Ribosomal RNA synthesis in Escherichia coli involves a transcription complex, in which RNA polymerase is modified by a signal element on the transcript, Nus factors A, B, E and G, ribosomal protein S4 and inositol mono-phosphatase SuhB. This complex is resistant to ρ-dependent termination and facilitates ribosomal RNA folding, maturation and subunit assembly. We show that SuhB directly binds the RNA signal element and the C-terminal AR2 domain of NusA, and we delineate the atomic basis of the latter interaction by macromolecular crystallography. The SuhB monomers are folded as an alternating stack of three pairs of α helices (helix pairs I–III) and two β sheets.

About 1600 Å2 of combined surface area are buried at the dimer interface. It has been suggested that wild type (wt) SuhB might form monomers, and that the R184A mutation stabilized the dimer state observed in the crystal structure of SuhBR184A. We therefore also crystallized wt SuhB alone and determined its structure at 2.25 Å resolution. Isolated wt SuhB crystallized with one monomer in an asymmetric unit, but a dimer essentially identical to the dimer seen with SuhBR184A (rmsd 0.56 Å for 482 pairs of common Cα atoms) and in the SuhB-NusAAR2 complex (rmsd 0.49 Å for 497 pairs of common Cα atoms) was formed by crystal symmetry. Moreover, SEC coupled to multi-angle light scattering confirmed that SuhB forms dimers under the chosen conditions in solution (experimental molecular mass: 60.7 kDa; calculated molecular mass for a SuhB dimer: 58.3 kDa).

> GAMAMHPMLNIAVRAARKAGNLIAKNYETPDAVEASQKGSNDFVTNVDKAAEAVIIDTIRKSYPQHTIITEESGELEGTDQDVQWVIDPLDGTTNFIKRLPHFAVSIAVRIKGRTEVAVVYDPMRNELFTATRGQGAQLNGYRLRGSTARDLDGTILATGFPFKAKQYATTYINIVGKLFNECADFRRTGSAALDLAYVAAGRVDGFFEIGLRPWDFAAGELLVREAGGIVSDFTGGHNYMLTGNIVAGNPRVVKAMLANMRDELSDALKR N-hydroxy-2-[(3S,5S,7S)-tricyclo[3.3.1.1~3,7~]dec-1-yl]acetamide | C12 H19 N O2 | 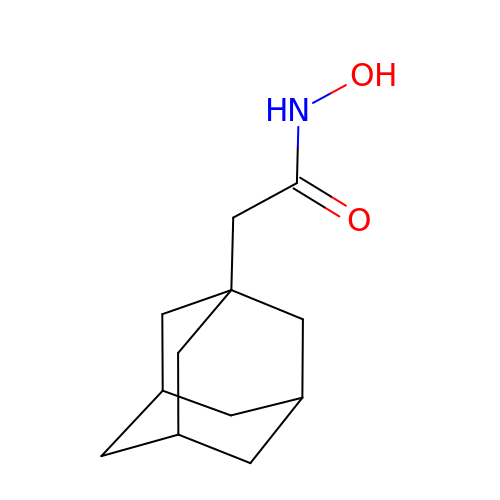JKZCKUGJZBWOQO-GOCCLTDMSA-N>[10x]MASTTRLVNDRKQLEQQVKDDARILADARGLNITTVANDSATGGQAIRNVGPNDEATIKALDNVIKQIEALSVIVNRSEKADDAQILGPNTYKQLLEHLFSPEENVYILLPIQAYTGGVIDRRDASFSNFAYSIASKLMMELSAATHNKIFTDYTRIAASALGPEISTEGMPLFSLIESLELTEAETSRLPVIQDSMVIQKSTATVGNAQQGISTINIKRVPFVGSAFQQVIDQLLWEYSTTSLTTKEQRRQRITEMVNDRRIMIQKLTLAEKPQVMRHVTTEINNDLFFKMSPVAQLYIYHLDRAFLDGVGFTPLAEKQQQLQLQLKTNILTANLIRSAINGMNTESNLEVAIKMMQAAQLHRASIEIAFPMNVSLSPEIIVQCFIVWMSIPEQLLSDRSNFIIAAVIWAGFSADDSYADIMRRSARASDRQNYDIIKAALSSRKFKLPRASTTLFDENEPVVRRYQIGRVYAPFPVDRYGSPVYSNCTKVELASDYNAEGFTIRKDDFRALQAVLRIDEDRAADMFTTLRIMISSIPAVWYDAEVVHYPHTAVELEQLAAYGLTGAYPRTNHSVDTIVKTVNNISATYSTIAQMLSTIDLDPTRYGTSESIDKFKIAWENVESVLNMEGNDFVKTIMYAYEDNFPKKDFYMMLKQIASDGQGAHPIAAAIDQLRTIVYREPERFGYIDSVILTHNPDVDTAYNRFFHLHPIVTNQPSNTIKNAQLWNEMRLEQQVEHIKAGPVRIIGPFHVTYNYLSEEEDMPATSHIIMKDNMILNDHLTFNFVKRERRNNKKRVSSFRYKAVEMYVAVRISRFQLEVLRDLHDLVRSRTYLDVSKSPLATTPIRVVEYVR;> MRIMAQRLKELQREIDKKKKERIAEAYLSSVEVTNSSPSLSKQDDALTLPKVSPFLDSTPFTTLHNSLYGQQIHSIDDELAQICKLEYELQTQIADEQITALKHFLTIRTGSPQEIQYVDKEWMKSNQHVPSFLGDVKLMFGDTAGKFRSTSKSVDSIHSITSDVQVTRKKQTRSQIRNSYRVQKKHKVQQPLKPNTLYVYKYKGLPRVVLRFVPKVDTTSNSNSSSASDSKKDKDAFSCDDLSPTWKYILTEAKRAFPDRSYSDCIHPMTWEEWLEENQDHVKVLTQYAHQLDYVTLLQDFNLYVSGGASRVRNIDMSTLPTSINVLDHFELYGDASMKEYVRSGEW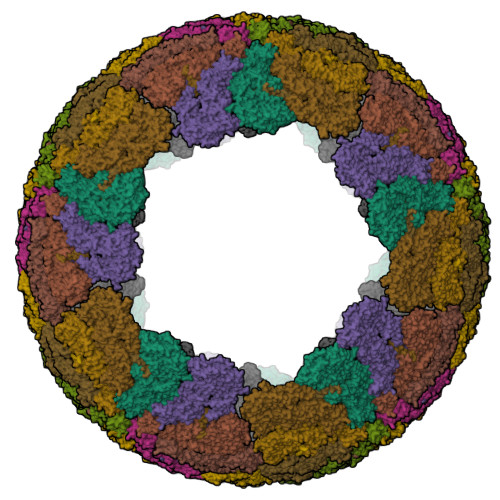YGLLREIEQEGMTVNESEKVFANPDTYVLNVKKYFLRRFQQEIASTGMTPLTDELLNIMFVHWNIIVTAEPKLQVIKDDLLKYYSRYGVDATFDYNMKRSEMTVVTRGHLLAHKVLECALRIVETIYTYDIQDETFKDILIDLGRLIMRDPIYGTTTVRDATTVMKQLMYTQGTQFRRIMFKKYDYSNFNEKLVLKGEQMTNEPPTLLATTHYEEMDKKRIDALIKANQRAGNILSQSSIERCRYTDSLDLVGDANRYFSALTTLEAVAGFASSDLLSGFIDSNESIEFTGTAHLRKLLYHSVREQITTLNTSTVPRPSLPKVLLSSAKDTASASIEPLTFRIYKTTPEYDGESLNLVESTVEMSTRQKKPNLMKAAEILRSTVTTNQEMIISGGTRAVQGGKGARAVYPTKQPYHIAGSLLFHKVDTIVNANKKYRGVSNKYGQGISNAIPHIGVPEIIAVSSDGMAICLALDVSAFDVAQKYTEADIELAMRDGFLDSEISMISGETVLERMNPADLANNLLTNTPPRYKYQTALGDIIILQHDNRSGVPWTGTQNDLVNVSNHHMAYDEYKKRVAELQRQGKISIDVNDKHHIVRVFGDDSTFIMTYDEPPSAEEVHLMCATFVESYQDTAGTLGFAINARKGMIGRYGSEYLKNSAIYGNIKSVNQVKFRGSEKSASYHFGVSEKVSMIRDITDLTITRGCDETRKWKYNLMMLPVDLTTRAGAFRMHNLCSIMTGVGKMYLGGTLNNKLIASYHGSSFGWNFDDNLIKTANSIGAISDSSYDAISTKITNLADFKDSQQRITRDIITSGRLPQHLNRYGKSNILRHILASAAMGPLSQIEKNVNAYNVVMGILNGKLEAPTVLERLNMGFKYVVMSDLKQDDYSPYSCQGLQYRRMLVHWGLNDSRITSFDPKGKLQHLLAKNSQILPIHFDIEFVYRLYLQAGTMGFLQVMSYYQLPDTLTHEMLAAVVALELQLGNDKYAVDMGVYSSQAGQIRINDALMDSIIQHRRGPPLPIIDRTLNRLLLHTYMLMFGLMGKSIDSTKIDPTLSWRAILESNDQRIAQLSELLTAV> AMHPRKDWYELTRATNWTPSYVTEEQLFPERMSGHMGIPLEKWESYDEPYKTSYPEYVSIQREKDAGAYSVKAALERAKIYENSDPGWISTLKSHYGAIAVGEYAAVTGEGRMARFSKAPGNRNMATFGMMDELRHGQLQLFFPHEYCKKDRQFDWAWRAYHSNEWAAIAAKHFFDDIITGRDAISVAIMLTFSFETGFTNMQFLGLAADAAEAGDYTFANLISSIQTDESRHAQQGGPALQLLIENGKREEAQKKVDMAIWRAWRLFAVLTGPVMDYYTPLEDRSQSFKEFMYEWIIGQFERSLIDLGLDKPWYWDLFLKDIDE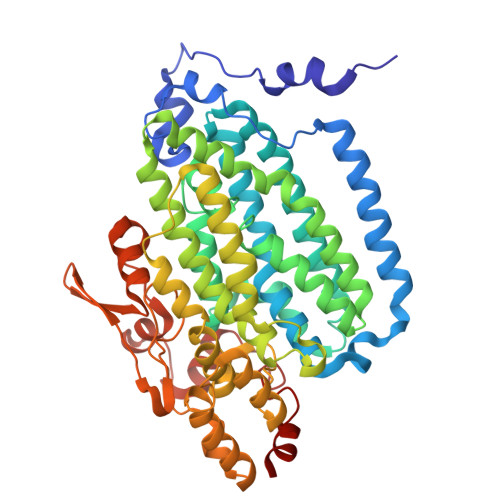LHHSYHMGVWYWRTTAWWNPAAGVTPEERDWLEEKYPGWNKRWGRCWDVITENVLNDRMDLVSPETLPSVCNMSQIPLVGVPGDDWNIEVFSLEHNGRLYHFGSEVDRWVFQQDPVQYQNHMNIVDRFLAGQIQPMTLEGALKYMGFQSIEEMGKDAHDFAWADKCK> FPTDDDDKIVGGYTCAANSIPYQVSLNSGSHFCGGSLINSQWVVSAAHCYKSRIQVRLGEHNIDVLEGNEQFINAAKIITHPNFNGNTLDNDIMLIKLSSPATLNSRVATVS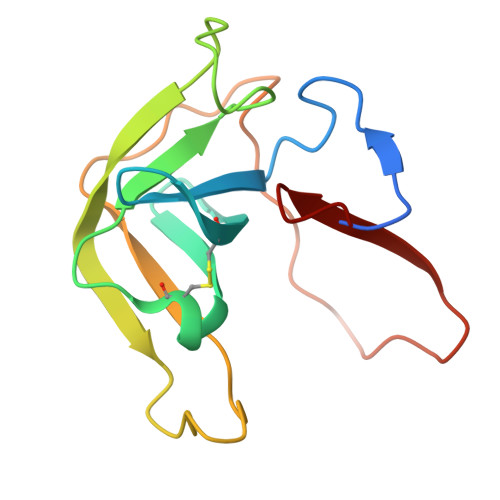LPRSCAAAGTECLISGWGNTK methyl 2-(5-methyl-2-phenyl-1,3-thiazol-4-yl)ethanoate | C13 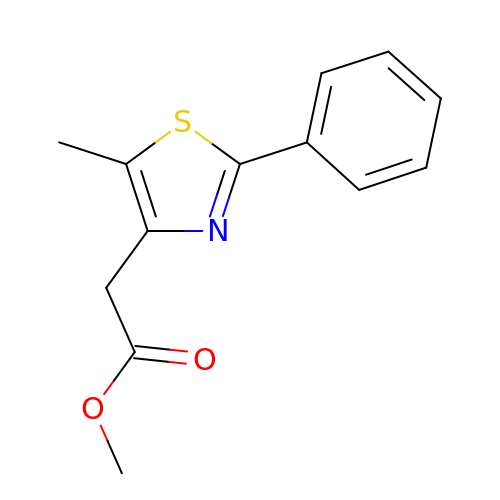H13 N O2 S | IGRGQWSVDTYHID-UHFFFAOYSA-N>[3x]GPMGKPARKGAEWKRFLKNNWVLLSTVAAVVLGITTGVLVREHSNLSTLEKFYFAFPGEILMRMLKLIILPLIISSMITGVAALDSNVSGKIGLRAVVYYFATTLIAVILGIVLVVSIKPGVTQKVGEIARTGSTPEVSTVDAMLDLIRNMFPENLVQAAFQQYKTKREEVKPPSDPEMTMTEESFTAVMTTAISKTKTKEYKIVGMYSDGINVLGLIVFALVFGLVIGKMGEKGQILVDFFNALSDATMKIVQIIMWYMPLGILFLIAGCIIEVEDWEIFRKLGLYMATVLTGLAIHSIVILPLIYFIVVRKNPFRFAMGMAQALLTALMISSSSATLPVTFRCAEENNQVDKRITRFVLPVGATINMDGTALYEAVAAVFIAQLNDLDLGIGQIITISITATSASIGAAGVPQAGLVTMVIVLSAVGLPAEDVTLIIA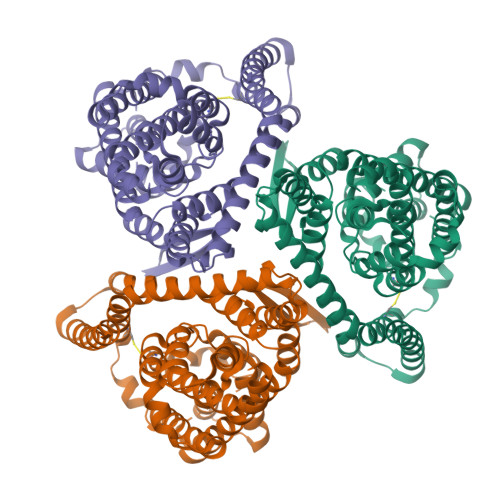VDCLLDRFRTMVNVLGDAFGTGIVEKLSKKELEQMDVSSEVNIVNPFALESTILDNEDSDTKKSYVNGGFAVDKSDTISFTQTSQF>MSKIEKLSILGVRSFGPHHPETIAFNTPLTLIVGYNGSGKTTVIECLKYATTGELPPNSTRNGAFIHDPDLVGEKEVRAQVKLSFRSTIGESYVVTRNIQLLVQRNNKRTQKTLEGSLLLRNNGERTVISTRVAELDKLVSEKLGVPPAILDAVIFCHQDDSLWPMSEPAALKKRFDEIFEAQKYTKVIENIRLLKKKKGDELKILKEREVQDKANKERAEKVDGGAGGAGGELDLKDAKAKYKETHIKVETTKAAIEDLGRGMAAVDHAIMQYHSKMMEQ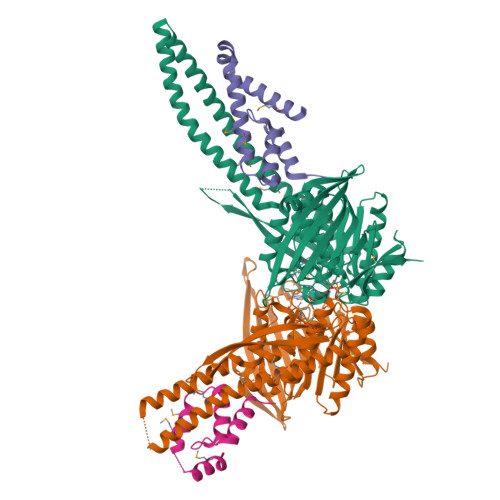INRTIAELWQSTYQGTDIDTIQIRSDVESTTSSDSGTRRNYNYRVSMVKGDTEMDMRGRCSAGQKVLASIIIRLALAESFCANCGLIALDEPTTNLDSDNIRSLAESLHGIIKARQAQGNLQLIVITHDEEFLKYMQCSDFCDDFYRVKRDEKQNSVIVRESITRITE[2x];>[2x]SDSISVDALVQEFFAQQSLKILPQAPFGDAVNQFVSKDDKHAVEMFVMDSLSSQVRGLLQLDDDKINEGLDSHIEDFRKVMEKNFLSGQQKQAQRRRRFKEKHHHHHH> MAHHGVSGLVGKLVTQLEVNCDADIFYKIVKHHEEVPNVIPHFFTGVQVTKGDGLVSGSIKEWNYVLEGKAMTAVEETTHADETRTLTHHITEGDAMKDYKKFDVIVETNPKPNGHGSVVTYSIVYEKINEDSPAPFDYLKFFHQNIVDMSAHICSSA

Several proteins from plant pathogenesis-related family 10 (PR10) are highly abundant in the latex of opium poppy and have recently been shown to play diverse and important roles in the biosynthesis of benzylisoquinoline alkaloids (BIAs). PR10-10 has been proposed to act as a noncatalytic BIA binding protein. We observed that an intermolecular disulfide bond between Cys59 and Cys155 is formed in the apo structure, while the binding of alkaloid compounds to the central hydrophobic pocket induces conformational changes that prevent the formation of this intermolecular disulfide bond.

To decouple ligand binding from disulfide-bond formation, each of the two highly conserved cysteine residues (Cys59 and Cys155) in PR10-10 was replaced with serine using site-directed mutagenesis. Crystal structures of the Cys59Ser mutant were determined in the presence of papaverine and in the absence of exogenous BIA compounds. Attempts to crystallize the Cys59Ser and Cys155Ser mutants of PR10-10 in the absence of BIA ligands surprisingly yielded crystals with the morphology characteristic of PR10-10 with bound BIA ligands. Data processing confirms that these crystals show C2221 space-group symmetry, and structure determination and refinement reveal a closed cap-loop conformation similar to the structures of PR10-10 with bound BIA ligands. Instead, each mutant protein crystallized in a ligand-bound conformation in the absence of exogenous alkaloid, with the appearance of electron density in the ligand-binding site corresponding to an unknown small molecule that presumably copurified with each protein. However, the higher quality of the electron density in this region allowed the modeling of the whole cap loop in PR10-10-Cys59Ser with a bound unknown ligand. Residues 33–36 in the α1 helix unwind and adopt a nonhelical backbone conformation to close off the BIA binding pocket. Our new crystal structures, from which the full cap loop is modeled, reveal that the side chain of Glu35 points into the BIA binding pocket after the C-terminal end of the α1 helix. The key cap-loop residues Glu35 and Val36, which contribute to the BIA binding pocket in the holo form, are shifted ∼4 Å into the BIA binding pocket in PR10-10-Cys59Ser compared with wild-type holo PR10-10, thereby decreasing the size of the pocket. Structural alignments showed that the smaller BIA binding pocket in PR10-10-Cys59Ser does not provide sufficient space for papaverine binding, specifically the position of main and side chain of Val36. The cap loop appears to be capable of adopting different conformations to accommodate the binding of different-sized ligands.>[4x]HFQLQWPGARGAFVANDEVYFCGAHNNVTTNRTDFPLDGSGFVSIKSGHAPYTVGAIISLETDADA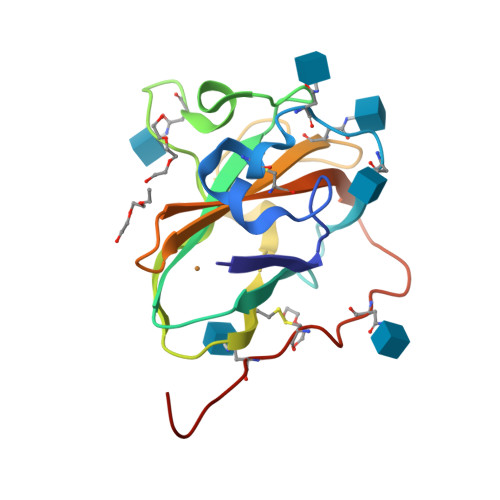WEDFKNSSGGDQIAIAYRQVDNSGTYCVPFNPSSLNIAGIQDGANATIQVVYTGGDGNLYQCADVTFRTTVANLNSSVCTNSTHHHHHH> D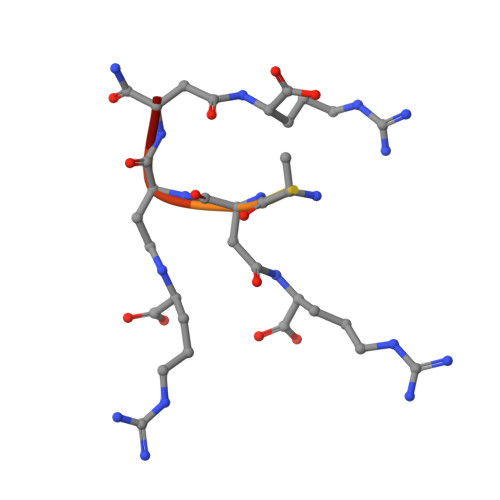DDDDDDDX To address this question, we chose to study transient receptor vanilloid member 1 (TRPV1), which is the receptor for vanilloids and noxious heat. TRPV1 is a homotetramer, where each protomer has an N-terminal cytosolic ankyrin repeat domain (ARD) and a transmembrane domain (TMD) of six transmembrane helices (S1-S6). The TMD is composed of a voltage sensor-like S1-S4 domain (VSLD), a pore domain (S5, the turret, the pore helix (PH), the selectivity filter (SF), the pore loop (PL), and S6), and the amphipathic TRP helix. Vanilloid binding at the S1-S4 domain allosterically acts upon the pore domain, driving pore opening.

Various strategies of 3D classification of the 4 °C dataset consistently resulted in three distinct classes with nearly equal particle distributions to overall excellent quality. For the three classes of RTx-TRPV1 at 4 °C, we assigned class I, class II, and class III according to the size of the pore opening (class I being the narrowest). Notably, the models from the 4 °C class II and 25 °C class A reconstructions have similar overall conformations (Cα r.m.s.d. ~0.6 Å), however local differences near the SF and the CD suggests that they represent two intermediate substates (see the analysis below). Compared to TRPV1C,RTx, the 4 °C intermediate state (TRPV1IC,RTx) exhibits rotation of the TRP domain while the C-terminal half of S6 (S6b) rotates and tilts away from the ion permeation pathway so that the diagonal distance between the side chains of I679 in the S6 gate is larger than 8 Å, consistent with an open conformation for the S6 gate. Rotation of S6b occurs at the π helical region between S6a and S6b. However, the SF of the 4 °C intermediate state adopts a nonconducting conformation, as there is minimal change at the SF with the diagonal distance between the side chains of M644 of 6.4 Å. Therefore, because both the SF and the S6 gate adopt conformations consistent with conductive states and the M644 flipped conformation is observed in the final open state (TRPV1O, RTx), we tentatively assign the model from the 25 °C class A reconstruction as an intermediate open state (TRPV1IO,RTx), while assigning the corresponding 4 °C class II reconstruction as an intermediate closed state (TRPV1IC,RTx). We reason that the two intermediate states at 4 °C and 25 °C represent substates in which their energetic and conformational differences are too small to be separated by cryo-EM 3D classification. Upon lowering the contour level of the cryo-EM density maps, we observe density for both M644 rotamers in both intermediate state 3D reconstructions, but the density corresponding to the non-conductive conformation predominates at 4 °C whereas the conductive conformation predominates at 25 °C, supporting our hypothesis.

>MEQRASLDSEESESPPQENSCLDPPDRDPNCKPPPVKPHIFTTRSRTRLFGKGDSEEASPLDCPYEEGGLASCPIITVSSVLTIQRPGDGPASVRPSSQDSVSAGEKPPRLYDRRSIFDAVAQSNCQELESLLPFLQRSKKRLTDSEFKDPETGKTCLLKAMLNLHNGQNDTIALLLDVARKTDSLKQFVNASYTDSYYKGQTALHIAIERRNMTLVTLLVENGADVQAAANGDFFKKTKGRPGFYFGELPLSLAACTNQLAIVKFLLQNSWQPADISARDSVGNTVLHALVEVADNTVDNTKFVTSMYNEILILGAKLHPTLKLEEITNRKGLTPLALAASSGKIGVLAYILQREIHEPECRHLSRKFTEWAYGPVHSSLYDLSCIDTCEKNSVLEVIAYSSSETPNRHDMLLVEPLNRLLQDKWDRFVKRIFYFNFFVYCLYMIIFTAAAYYRPVEGLPPYKLKNTVGDYFRVTGEILSVSGGVYFFFRGIQYFLQRRPSLKSLFVDSYSEILFFVQSLFMLVSVVLYFSQRKEYVASMVFSLAMGWTNMLYYTRGFQQMGIYAVMIEKMILRDLCRFMFVYLVFLFGFSTAVVTLIEDGKNNSLPMESTPHKCRGSACKPGNSYNSLYSTCLELFKFTIGMGDLEFTENYDFKAVFIILLLAYVILTYILLLNMLIALMGETVNKIAQESKNIWKLQRAITILDTEKSFLKCMRKAFRSGKLLQVGFTPDGKDDYRWCFRVDEVNWTTWNTNVGIINEDPGNCEGVKRTLSFSLRSGRVSGRNWKNFALVPLLRDASTRDRHATQQEEVQLKHYTGSLKPEDAEVFKDSMVPGEKENSLEVLFQGPDYKDDDDKAHHHHHHHHHH[4x]The GH5 arabinoxylanase (CtXyl5A) derived from Clostridium thermocellum displays an absolute requirement for xylans that contain Araf side chains. In this enzyme, the key specificity determinant is the Araf appended to O3 of the Xylp bound in the active site (−1 subsite). The dockerin domain recruits the enzyme into the cellulosome, a multienzyme plant cell wall degrading complex presented on the surface of C. thermocellum.

To understand the structural basis for the biochemical properties of CtXyl5A, the crystal structure of the enzyme with ligands that occupy the substrate binding cleft and the critical −2* subsite were sought. The data presented in Fig. 3A show the structure of the CtXyl5A derivative CtGH5-CtCBM6 in complex with arabinose bound in the −2* pocket. Interestingly, the bound arabinose was in the pyranose conformation rather than in its furanose form found in arabinoxylans. O1 was facing toward the active site −1 subsite, indicative of the bound arabinose being in the right orientation to be linked to the xylan backbone via an α-1,3 linkage. As discussed on below, the axial O4 of the Arap did not interact with the −2* subsite, suggesting that the pocket might be capable of binding a xylose molecule. Analysis of the three structures showed that O1, O2, O3, and the endocyclic oxygen occupied identical positions in the Arap, Araf, and Xylp ligands bound in the −2* subsite and thus made identical interactions with the pocket. O1 makes a polar contact with Nδ2 of Asn139, O2 is within hydrogen bonding distance with Oδ1 of Asn139 and the backbone N of Asn135, and O3 interacts with the N of Gly136 and Oϵ2 of Glu68. Although O4 of Arap does not make a direct interaction with the enzyme, O4 and O5 of Xylp and Araf, respectively, form hydrogen bonds with Oϵ1 of Glu68. Finally Tyr92 makes apolar parallel interactions with the pyranose or furanose rings of the three sugars. The mutants E68A, Y92A, and N139A were all inactive, demonstrating the importance of the interactions of these residues with the substrate and reinforcing the critical role the −2* subsite plays in the activity of the enzyme.

> MASSPQRGRPRLNAARTTFVGDNGQPLRGPYTSTEWTAAAPYDQIARVKELGFNAVHLYAECFDPRYPAPGSKAPGYAVNEIDKIVERTRELGLYLVITIGNGANNGNHNAQWARDFWKFYAPRYAKETHVLYEIHNEPVAWGPPYSSSTANPPGAVDMEIDVYRIIRTYAPETPVLLFSYAVFGGKGGAAEALKDIRAFNKAVFGNENAVWTNEAVAFHGYAGWQETTIAVEELLKAGYPCFMTEYAGGAWGSGMGGLDVELTYELERLGVSWLTFQYIPPTGVSDDVTKPEYFSALVENSGLSWTPDYGNWPAARGVYGNGGLARETATWINNFLTGTTRIEAEDFDWGGNGVSYYDTDSVNVGGQYRPDEGVDIEKTSDTGGGYNVGWISEGEWLEYTIRVRNPGYYNLSLRVAGISGSRVQVSFGNQDKTGVWELPATGGFQTWTTATRQVFLGAGLQKLRINALSGGFNLNWIELSPILEHHHHHH>MGRKKIQITRIMDERNRQVTFTKRKFGLMKKAYELSVLCDCEIALIIFNSSNKLFQYASTDMDKVLLKYTEYSEPHESRTNTDILETLKRREHR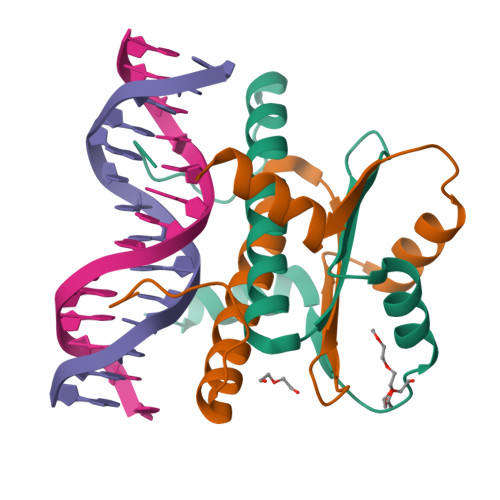G[4x]> SDTHIFIIMGASGDLAKKKIYPTIWWLFRDGLLPENTFIVGYARSRLTVADIRKQSEPFFKATPEEKLKLEDFFARNSYVAGQYDDAASYQRLNSHMNALHLGSQANRLFYLALPPTVYEAVTKNIHESCMSQIGWNRIIVEKPFGRDLQSSDRLSNHISSLFREDQIYRIDHYLGKEMVQNLMVLRFANRIFGPIWNRDNIACVILTFKEPFGTEGRGGYFDEFGIIRDVMQNHLLQMLCLVAMEKPASTNSDDVRDEKVKVLKCISEVQANNVVLGQYVGNPDGEG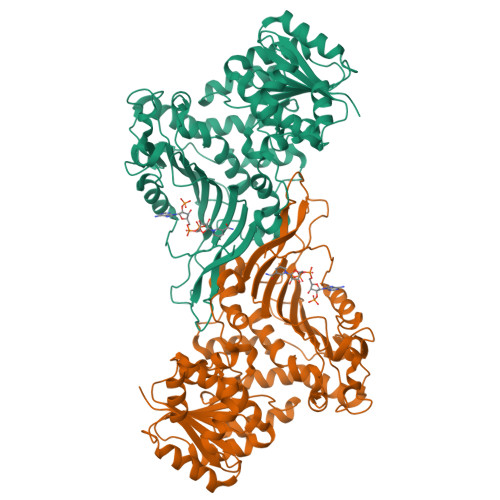EATKGYLDDPTVPRGSTTATFAAVVLYVENERWDGVPFILRCGKALNERKAEVRLQFHDVAGDIFHQQCKRNELVIRVQPNEAVYTKMMTKKPGMFFNPEESELDLTYGNRYKNVKLPDAYERLILDVFCGSQMHFVRSDELLEAWRIFTPLLHQIELEKPKPIPYIYGSRGPTEADELMKRVGFQYEGTYKWVNPH3-AMINOOXY-1-AMINOPROPANE | C3 H10 N2 O | 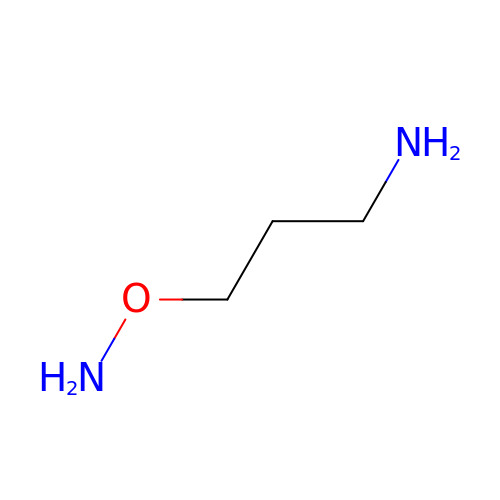VSZFWDPIWSPZON-UHFFFAOYSA-N> MRVILNTGRTIWQGQAIESGKDLKMYVDAAA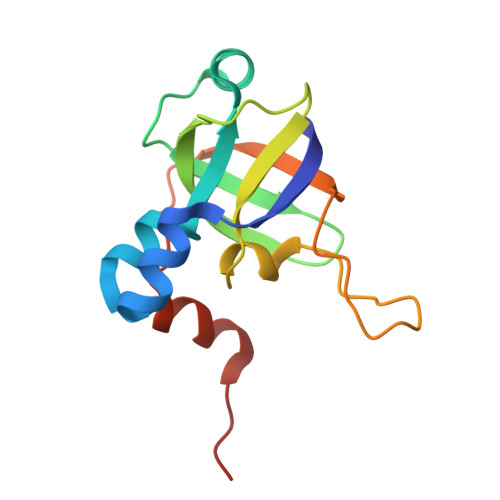IIQMNPEMMKQLGIAEGDNVKVISEYGDVVVKAVEAKEPLPEGMVYIPMGPWANRVIRPYTDSTATPSFKNIPVEIIPTDEEVLDMPTLMKVYGKVGQI>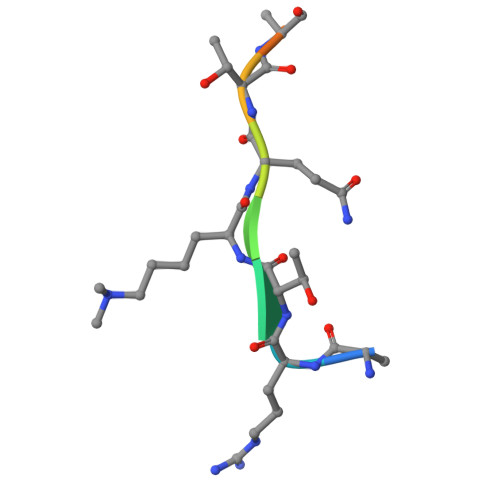 ARTKQTARKY> HGYMSFPIARQRRCSMESFWYPTNGDGITDPMCRAAYQYVYDKVLDETGSTTDAISAAQYEFQQDNEYAALAGPDYWDKCHITQQVVPNYLCAAGAHSWSNPFGDKSGVDISGSWRPTVIPLSDNHQVSVPLELEFCPTAVHEPSYYEVYITKPSF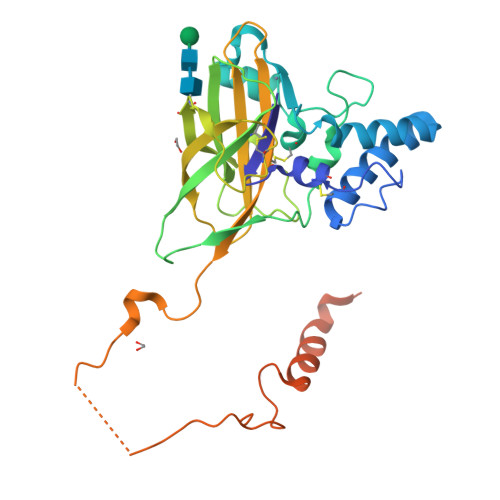NVFIDRVVWGNLDLIYNDTVPLDPRLPYSICDADLVYRFTVPIPIRQSQAVLYVRWQRLDPVGEGFYNCVDINFDYNNGPDDEDIIVPDVEGGLLPNQCASTFNYNEGVPGFDTEEYYKYMYESLRFNRYNTNTCSSRDYGKQKWHRRHHHQYVYNK> DFQSESYKDAYSRINAIVIEGEQEAFDNYNRLAEMLPDQRDELHKLAKMEQRHMKGFMACGKNLSVTPDMGFAQKFFERLHENFKAAAAEGKVVTCLLIQSLIIECFAIAAYNIYIPVADAFARKITEGVVRDEYLHRNFGEEWLKANFDASKAELEEANRQNLPLVWLMLNEVADDARELGMERESLVEDFMIAYGEALENIGFTTREIMRMSAYGLAAV;> LDFQSESYKDAYSRINAIVIEGEQEAFDNYNRLAEMLPDQRDELHKLAKMEQRHMKGFMACGKNLSVTPDMGFAQKFFERLHENFKAAAAEGKVVTCLLIQSLIIECFAIAAYNIYIPVADAFARKITEGVVRDEYLHRNFGEEWLKANFDASKAELEEANRQNLPLVWLMLNEVADDARELGMERESLVEDFMIAYGEALENIGFTTREIMRMSAYGLAAV

Cyanobacterial aldehyde-deformylating oxygenase (cADO), which catalyzes the conversion of Cn fatty aldehyde to its corresponding Cn-1 alk(a/e)ne, is a key enzyme in that pathway. Cyanobacterial aldehyde-deformylating oxygenase (cADO) belongs to the superfamily of ferritin-like di-iron proteins and contains a di-iron center. To gain insights into the reaction catalyzed by cADO, we determined structures of wild type ADO from Synechococcus elongates PCC7942 (Se) with different treatment (WT0, no treatment; WT1, co-crystallized with iron; WT-HP, soaked in H2O2), and solved the structures of two SeADO mutants (Y122F and F86YF87Y). SeADO belongs to the di-iron protein family, with conserved sequence of two EX28-29EX2H motifs, in which six conservative amino acids from four helices (Glu32 from helix H1, Glu115 from helix H4, Glu60 & His63 from helix H2, and Glu144 & His147 from helix H5) act as metal ligands.

Following the analysis of the extracts together with the observed electron densities, we built a long-chain fatty acid (Lox) into the structure of WT-HP, and a long-chain fatty alcohol (Lred) into three other structures. On the basis of these observations, we propose that the Lred ligand may represent the real substrate, namely fatty aldehyde, because of the similarity in their chemical structures. In the WT1 structure, a Lred ligand, which was proposed to mimic the substrate aldehyde, was modeled in the substrate channel according to the electron density. The ligand approaches the di-iron cluster from the opposite side of His147, with its head-group binding directly to the Fe2 atom. This coordination mode suggests that Fe2 is the preferred iron for substrate binding. The water molecule, located near the di-iron site in the Y122F structure, is displaced by the head group of the Lred ligand. The residue Glu144, which is located in helix H5, changes its rotamer and is not coordinated with either iron atoms. In addition, E115 alters its mode of Fe2 coordination, from bidentate to monodentate, while other four iron-coordinating residues stay unchanged, resulting in a distorted tetrahedral coordination of both Fe1 and Fe2. The structure of WT1 is likely to represent the state where the enzyme is bound with substrate. The structural comparison between WT1 and Y122F implied that the swing of Glu144 might be induced by ligand binding, thus enabled us to visualize the conformational change coupled with substrate binding in cADO active site for the first time.>[2x]MSALFEPYTLKDVTLRNRIAIPPMCQYMAEDGLINDWHQVHYASMARGGAGLLVVEATAVAPEGRITPGCAGIWSDAHAQAFVPVVQAIKAAGSVPGIQIAHAGRKASANRPWEGDDHIGADDARGWETIAPSAIAFGAHLPNVPRAMTLDDIARVKQDFVDAARRARDAGFEWIELHFAHGYLGQSFFSEHSNKRTDAYGGSFDNRSRFLLETLAAVREVWPENLPLTARFGVLEYDGRDEQTLEESIELARRFKAGGLDLLSVSVGFTIPETNIPWGPAFMGPIAERVRREAKLPVTSAWGFGTPQLAEAALQANQLDLVSVGRAHLADPHWAYFAAKELGVEKASWTLPAPYAHWLERYRRPHHHHHH

The biocatalytic reduction of the oxime moiety to the corresponding amine group has only recently been found to be a promiscuous activity of ene-reductases transforming α-oximo β-keto esters. By studying the crystal structures of enzyme oxime complexes, analyzing molecular dynamics simulations, and investigating biocatalytic cascades and possible intermediates, we obtained evidence that the reaction proceeds via an imine intermediate and not via the hydroxylamine intermediate. To gain more insight into the reaction pathway, we determined the crystal structures of the two enzymes OPR3 and XenA in complex with the oxime substrates 1a–c, either by co-crystallization or by soaking. All the crystal structures obtained had a high resolution (1.9–1.35 Å) and showed clear electron density features for the oximes.

In general, XenA structures showed a better-defined electron density for the substrate when prepared by soaking, while for OPR3, clearer results were obtained by co-crystallization. The propanoyl moiety of oxime 1b points into this cavity and is likely stabilized by hydrophobic interactions. Substrates with an acetyl moiety (such as oximes 1a and 1c) give the non-productive binding mode described above. Comparable experimental pKa values are reported for chemically similar oximes and for the 8-hydroxycoumarin and para-hydroxybenzaldehyde. Substrates of ene-reductases usually bind with the hydride-receiving atom within van der Waals distance from the N5 of the flavin and with an enzyme-dependent angle between the flavin N10–N5 axis and the atom receiving the hydride. In the cases mentioned above, none of these criteria are satisfied, and the binding modes very likely correspond to catalytically non-active complexes. Thus, we will refer to it as the “non-productive binding mode”. The calculated high Kd for oxime 1b clearly indicates this enzyme’s low affinity for the substrate and might explain why this enzyme performed poorly in the biotransformation of the other oximes in our previous work.>[8x]SNAMKILVDENMPYARELFSRLGEVKAVPGRPIPVEELNHADALMVRSV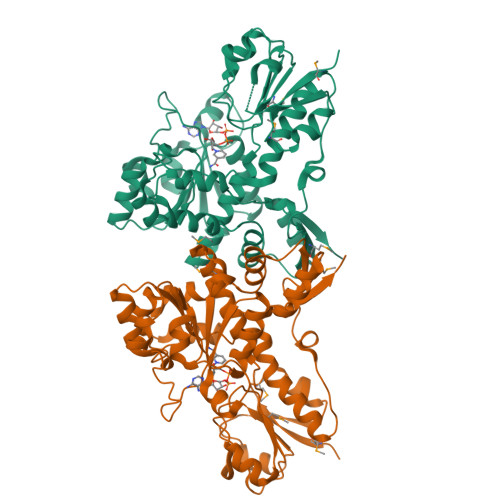TKVNESLLSGTPINFVGTATAGTDHVDEAWLKQAGIGFSAAPGCNAIAVVEYVFSALLMLAERDGFSLRDRTIGIVGVGNVGSRLQTRLEALGIRTLLCDPPRAARGDEGDFRTLDELVQEADVLTFHTPLYKDGPYKTLHLADETLIRRLKPGAILINACRGPVVDNAALLARLNAGQPLSVVLDVWEGEPDLNVALLEAVDIGTSHIAGYTLEGKARGTTQVFEAYSAFIGREQRVALETLLPAPEFGRITLHGPLDQPTLKRLAHLVYDVRRDDAPLRKVAGIPGEFDKLRKNYLERREWSSLYVMCDDETAAALLCKLGFNAVHHPAH N-(2-aminoethyl)-Nalpha-benzoyl-L-phenylalaninamide 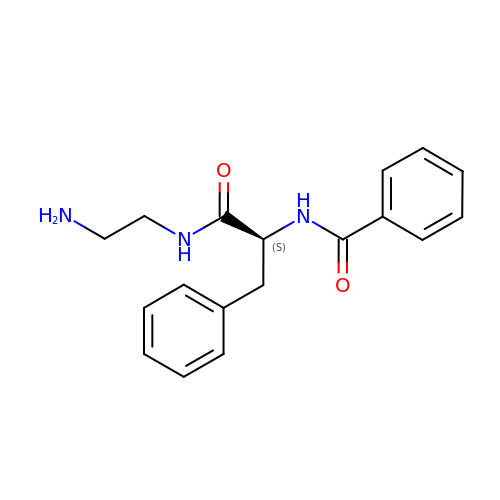| C18 H21 N3 O2 | WNPRWIUDHVJPCD-INIZCTEOSA-N> TAFLWAQNRNGLIGKD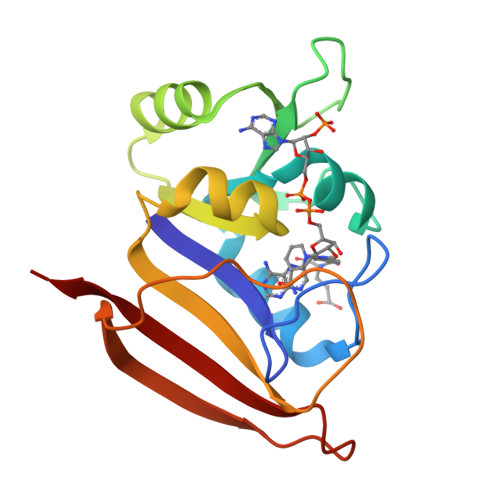GHLPWHLPDDLHYFRAQTVGKIMVVGRRTYESFPKRPLPERTNVVLTHQEDYQAQGAVVVHDVAAVFAYAKQHLDQELVIAGGAQIFTAFKDDVDTLLVTRLAGSFEGDTKMIPLNWDDFTKVSSRTVEDTNPALTHTYEVWQKKA>[2x]MKELIYIEEPSILFAHGQKCTDPRDGLALFGPLNQIYGIKSGVVGTQKGLQIFKSYLDKIQKPIYNHNNITRPMFPGFEAVFGCKWESQNIVFKEITDEEIRRYLFNASTHKRTYDLVTLFNDKIITANKNDEERVDVWFVIVPEEIYKYCRPNSVLPNELVQTKSLISKSKAKSFRYTPTLFEEFNKKLKEVEKEAKTYNYDAQFHDQLKARLLEHTIPTQILRESTLAWRDFKNTFGAPIRDFSKIEGHLAWTISTAAYYKAGGKPWKLGDIRPGVCYLGLVYKKIEKSKNPQNACCAAQMFLDNGDGTVFKGEVGPWYNPEKGEYHLKPKEAKALLTQALES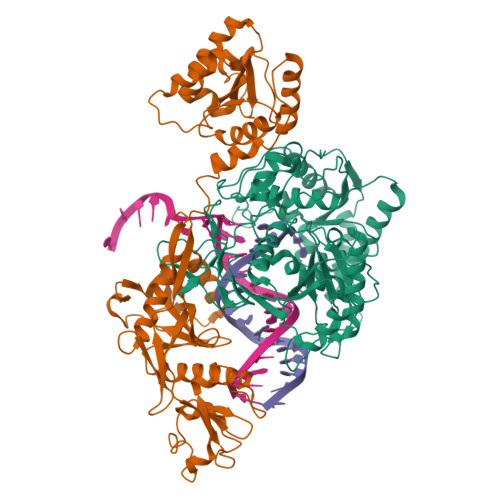YKEQNKSYPKEVFIHARTRFNDEEWNAFNEVTPKNTNLVGVTITKSKPLKLYKTEGAFPIMRGNAYIVDEKKAFLWTLGFVPKLQSTLSMEVPNPIFIEINKGEAEIQQVLKDILALTKLNYNACIYADGEPVTLRFANKIGEILTASTEIKTPPLAFKYYI;>MRNKIFISHATPEDDDFTRWLSLKLIGLGYEVWCDILFLDKGVDFWSTIEKEIRENTCKFLIVSSTAGNKREGVLKELAVATKVKKHLQDDMFIIPLAIDENLSYDDINIEIVRLNAIDFKKSWAKGLQDLLDAFEKQNVPKKPPDHSKSNLLYQQIFLHDKQAIEKEETYDSNWFPIISFPNELRFHRYDWRLPKQFDVRTLAFPAIRYKEYLCTFAWEYDFIHQLPKTETYNGQESIRISTSDILSGRYDTDFIRNYECQRLIVQLINKAFELRMKDKNVREYQMSKTFAYWIEKGKLEKDKFEKIKLVGKQKNKYWHFGISAAGKLYPSPVLMVSSHIIFTMDGINLIKSKSIQHSSRRKQGKNWWNDKWREKLLAFIRFLSDDQNAIYLNVGSEEKILISNKPLKFFGKMSYVTPSE[2x]>[2x]VPACTVSNTTVDWQDVEIQTLSQNGNHEKEFTVNMRCPYNLGTMKVTITATNTYNNAILVQNTSNTSSDGLLVYLYNSNAGNIGTAITLGTPFTPGKITGNNADKTISLHAKLGYKGNM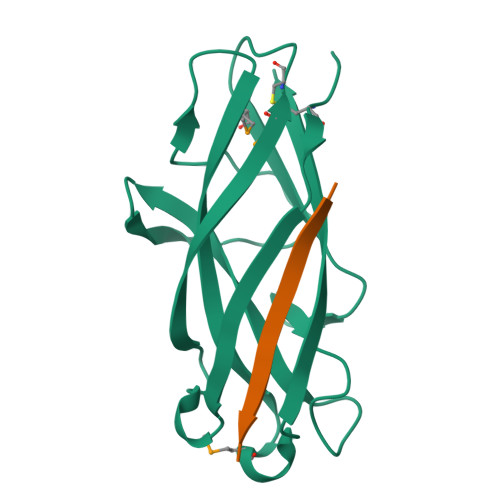QNLIAGPFSATATLVASYS;>[2x]SDVAFRGNLLD>[2x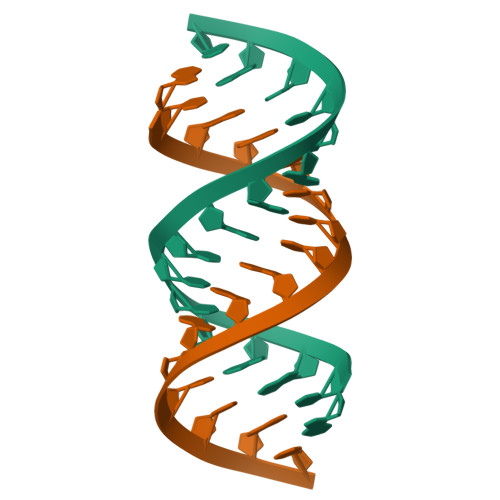]GCAGACUUAAAUCUGC>LVPNDTRYSEQWGYASGVGGANLPKAWDITTGSDKVVVAVVDTGYRPHADLAANILPGYDFISDPDSANDGNGRDNNAADPGDWVTQQEVDDPNGPFYRCQLDQFGNTFASNSSWHGTHVAGTIGAVSNNGTGVAGISWKGKILPVRVLGKCGGTLSDIADGMRWAAGLSVPGAPANPNPASVLNFSLGGGGSCSRTYQNAINAVVAKGATVVVAAGNEASPVSSSQPANCQNVIAVAATDINGRRASFTNTGSLVKIAAPGVNILSTLNSGTKSPAADSYASYNGTSMATPHVAGTVALMLAANGSLTPSQILQKLQASARPFPSGSGCSTSTCGAG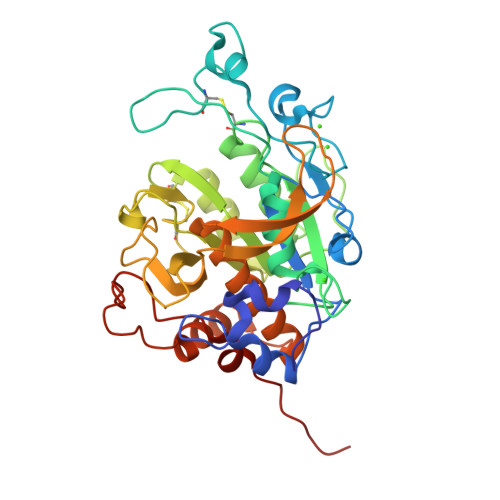LLDAGAAVNAARQHHHHHH[2x]>MALAEADDGAVVFGEEQEALVLKSWAVMKKDAANLGLRFFLKVFEIAPSAKQMFSFLRDSDVPLEKNPKLKTHAMSVFVMTCEAAAQLRKAGKVTVRETTLKRLGATHLRYGVADGHFEVTGFALLETIKEALPADMWSLEMKKAWAEAYSQLV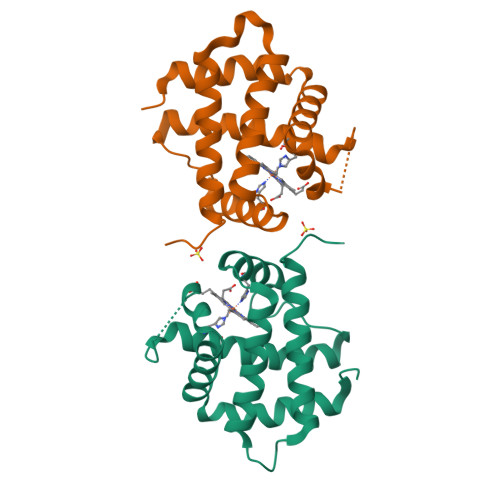AAIKREMKPDA[4x]>[2x]MAPPLVVVGSANADIYVEIERLPKEGETISAKTGQTLAGGKGANQAACGAKLMYPTYFVGRLGEDAHGKLIAEALGDDGCGVHLDYVRSVNNEPTGHAVVMLQSDGQNSIIIVGGANMKAWPEIM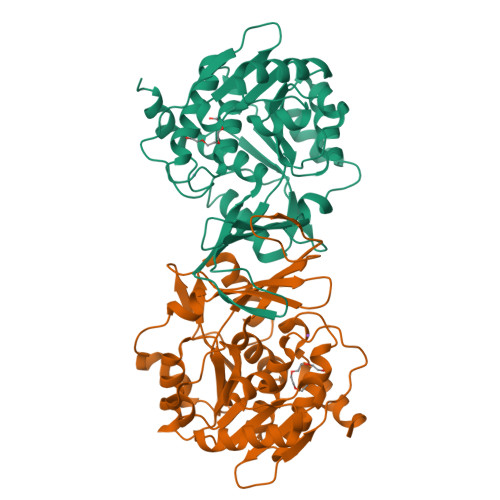SDDDLEIVRNAGIVLLQREIPDSINIQVAKAVKKAGVPVILDVGGMDTPIPNELLDSIDILSPNETELSRLTGMPTETFEQISQAVAKCHKLGVKQVLVKLGSKGSALFIQGEKPIQQSIIPAAQVVDTTGAGDTFTAAFAVAMVEGKSHEECLRFAAAAASLCVQVKGAIPSMPDRKSVLKLLKFSI(azepan-1-yl)(2H-1,3-benzodioxol-5-yl)methanone 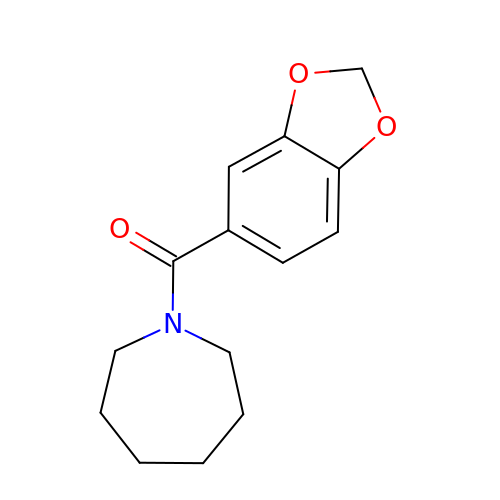| C14 H17 N O3 | ABPXISKFLMGPJG-UHFFFAOYSA-N> DAPESWDWSKKGVITKVKFQGQCGSGWAFSATGAIEAAHAIATGNLVSLSEQELIDCVDESEGCYNGWHYQSFEWVVKHGGIASEADYPYKARDGKCKANEIQDKVTIDNYGVQILSNESTESEAESSLQSFVLEQPISVSIDAKDFHFYSGGIYDGGNCSSPYGINHFVLIVGYGS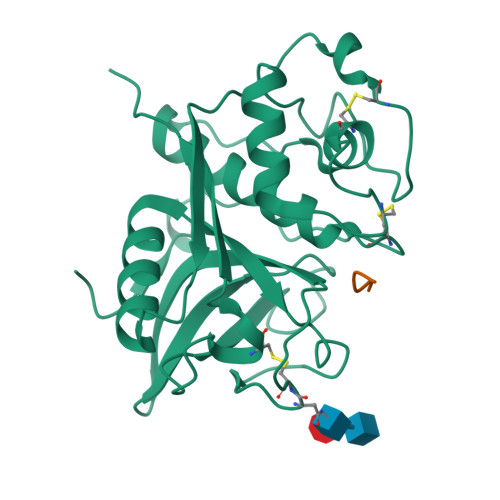EDGVDYWIAKNSWGEDWGIDGYIRIQRNTGNLLGVCGMNYFASYPIIEKSETLKFGRVKADPRVEHSPL;> KASVG> MAHHHHHHMEKVRVRFAPSPTGPLHLGGVRTALYDYLFAKHNGGDFILRIEDTDTQRYVPGSEEYIMEALEWIGMVPDESPKHGGPYAPYRQSERRDIYDRYTEQILKTDYAYLAFDTPEELDQIRAEFEARGDVFAYNYETRNRLRNSISLPEEEVKKLLEEKTPYVIRFKMPLDRIINLNDIIRGKFSVNTNTLDDKVLVKNDGMPTYHFANIIDDHEMKITHVIRGEEWLPSMALHVLLYEAMGWDAPEFAHLSLILKPEGKGKLSKRDGDKFGFPVFPLNFTDPATGNTSAGYREEGYLPEAFINMVAMLGWSPADNKEIVSMDEMIKEFDLNKVHKAGARFSAEKAKWFNQQYLQLMSNEAILPEFKKVLAENNVEVSDEKAL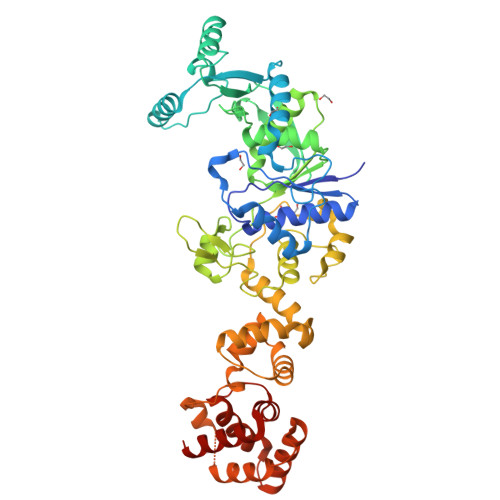KIIGLMKERATFVKDIYNDGKFFFHAPESFDEKASKKAWSPETAVLMQELTEAISSLDFKAEIIKESIHHLAEAKGLGMGKVMMPLRLSLVGELKGPDVPDLMEMIGKEETISRINKAIETLK> TSSANE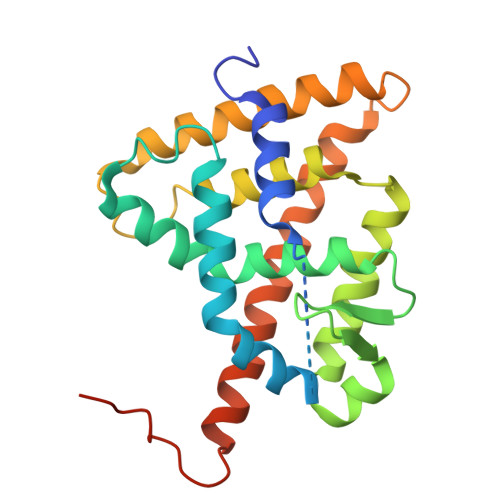DMPVERILEAELAVEPKTETYVEANMGLNPSSPNDPVTNICQAADKQLFTLVEWAKRIPHFSELPLDDQVILLRAGWNELLIASFSHRSIAVKDGILLATGLHVHRNSAHSAGVGAIFDRVLTELVSKMRDMQMDKTELGCLRAIVLFNPDSKGLSNPAEVEALREKVYASLEAYCKHKYPEQPGRFAKLLLRLPALRSIGLKCLEHLFFFKLIGDTPIDTFLMEMLEAPHQMT BCL-2 is the founding member of the pro-survival class of proteins that includes BCL-XL, BCL-W, A1/BFL-1 and MCL-1. They exert their pro-survival function by binding and restraining related members of a family of pro-apoptotic proteins—the sensors of cellular stress (the BH3-only proteins) and the effectors of apoptosis (BAX and BAK). Four or more hydrophobic amino acids on successive helical turns within the BH3 motif engage complementary pockets (P1 through P4) in this surface groove of pro-survival proteins. Venetoclax competes with pro-apoptotic BH3 motifs for BCL-2 binding, releasing pro-apoptotic proteins and allowing apoptosis in cells primed for death.

We have now crystallised and determined the structure of venetoclax bound to BCL-2 at high resolution. We obtained crystals of BCL-2 in complex with venetoclax that diffracted to high resolution (1.62 Å) in the space group P212121 with one molecule in the asymmetric unit. The electron density for the drug was well defined and the binding pose was in general agreement with the published structures of ABT-263 and compound 1, with the 4-chlorophenyl (CP) bound in the BCL-2 P2 pocket, the piperazine bridging the P2 and P4 pockets over residue F104 and the azaindole substitution bound in the BCL-2 P4 pocket. It was possible to model two distinct conformations with the 4–4-dimethylcyclohex-1-ene (4DM) ring flipping at the 4 and 5 positions above the BCL-2 P2 pocket and the benzamide (BA) acyl oxygen adopting two conformations above the BCL-2 P4 pocket. Notably, the orientation of the moiety inserted into the P2 pocket is subtly different in venetoclax compared to ABT-263 and compound 1 structures. The structure reveals subtle differences between the binding of the drug relative to the published analogues, which would not have been predicted based on the previous structures. Venetoclax selectively inhibits BCL-2, thereby promoting apoptosis in cells refractory to conventional apoptotic cues.

> MAHAGRTGYDNREIVMKYIHYKLSQRGYEWDAGDDVEENRTEAPEGTESEVVHLTLRQAGDDFSRRYRRDFAEMSSQLHLTPFTARGRFATVVEELFRDGVNWGRIVAFFEFGGVMCVESVNREMSPLVDNIALWMTEYLNRHLHTWIQDNGGWDAFVELYGPSMR> MDGALINSVLYVSPRNGAHYFVELTEKHLLAFEMLNSMCLLENYDHVLLFLECQFGKSHNLAVIPFDIILVLFTLSTLSEYYKEPILRANDPYNTSRETLSRRALKLLQKYLAILKEFDSEQYNLYDLELLRCQFFLAIDTLTPKKQKWGFDRFRRTKSESGVTYRQNASVDPELDQAKTFKNPYRSYISCLEQRNTILGNRLLNLKLNEPGEFINMILWTLSNSLQESTPLFLSSHEIWMPLLEILIDLFSCRQDYFIQHEVAQNVSKSLFVQRLSESPLAVFFESLNTRNFANRFSEYVFLNCDYKLPSDNYATPVHPVYNGENTIVDTYIPTIKCSPLYKSQKSLALRRKLIGSCFKLLLRVPDGHRLITPRIVADDVIQGISRTLASFNDILQFKKFFMTENLSQESYFIPLLAEGTLSEILKDTQECVVILTLVENLSDGVSFCNEVIGLVKSKCFAFTEQCSQASYEEAVLNIEKCD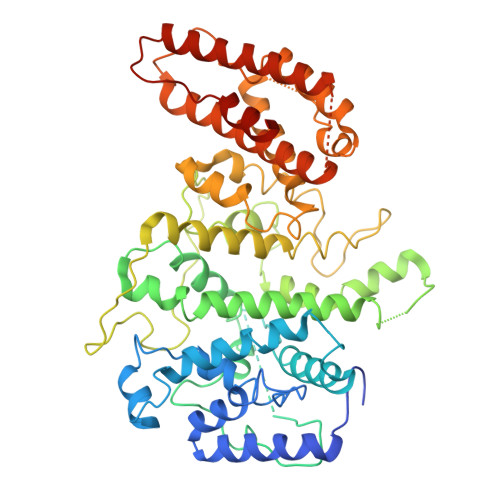VCLLVLLRYLLHLIGTEAILDAKEQLEMLHAIEKNDSGRRQWAKALNLGNDPPLLYPIVSQMFGVHDKSVIIE> PISPIETVPVKLKPGMDGPKVKQWPLTEEKIKALVEICTEMEKEGKISKIGPENPYNTPVFAIKKKDSTKWRKLVDFRELNKRTQDFWEVQLGIPHPAGLKKNKSVTVLDVGDAYFSVPLDEDFRKYTAFTIPSINNETPGIRYQYNVLPQGWKGSPAIFQSSMTKILEPFKKQNPDIVIYQYMDDLYVGSDLEIGQHRTKIEELRQHLLRWGLTTPDKKHQKEPPFLWMGYELHPDKWTVQPIVLPEKDSWTVNDIQKLVGKLNWASQIYPGIKVRQLCKLLRGTKALTEVIPLTEEAELELAENREILKEPVHGVYYDPSKDLIAEIQKQGQGQWTYQIYQEPFKNLKTGKYARMRGAHTNDVKQLTEAVQKITTESIVIWGKTPKFKLPIQKETWETWWTEYWQATWIPEWEFVNTPPLVKLWYQLEKEPIVGAETFYVDGAANRETKLGKAGYVTNKGRQKVVPLTNTTNQKTQLQAIYLALQDSGLEVNIVTDSQYALGIIQAQPDKSESELVNQIIEQLIKKEKVYLAWVPAHKGIGGNEQVDKLVSAGIRKIL;> PISPIETVPVKLKPGMDGPKVKQWPLTEEKIKALVEICTEMEKEGKISKIGPENPYNTPVFAIKKKDSTKWRKLVDFRELNKRTQDFWEVQLGIPHPAGLKKNKSVTVLDVGDAYFSVPLDEDFRKYTAFTIPSINNETPGIRYQYNVLPQGWKGSPAIFQSSMTKILEPFKKQNPDIVIYQYMDDLYVGSDLEIGQHRTKIEELRQHLLRWGLTTPDKKHQKEPPFLWMGYELHPDKWTVQPIVLPEKDSWTVNDIQKLVGKLNWASQI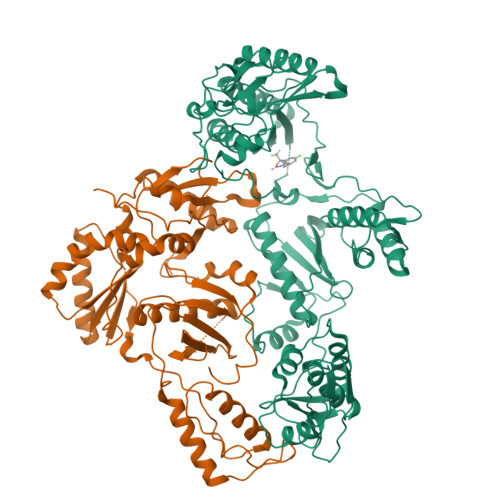YPGIKVRQLCKLLRGTKALTEVIPLTEEAELELAENREILKEPVHGVYYDPSKDLIAEIQKQGQGQWTYQIYQEPFKNLKTGKYARMRGAHTNDVKQLTEAVQKITTESIVIWGKTPKFKLPIQKETWETWWTEYWQATWIPEWEFVNTPPLVKLWY N-[4-(2-oxopyrrolidin-1-yl)phenyl]-2-(pyridin-2-yl)pyrimidine-5-carboxamide | C20 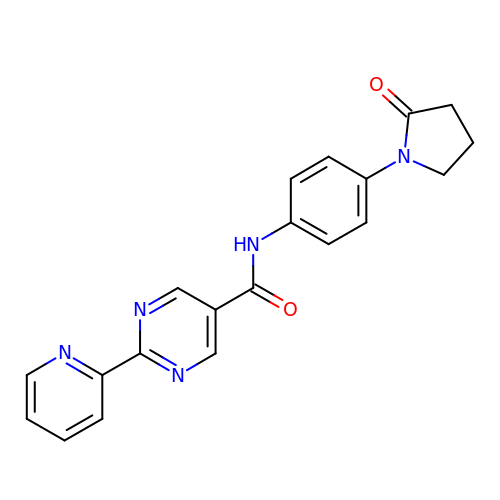H17 N5 O2 | MYYXEGDPWAHVAZ-UHFFFAOYSA-N Efficient egress by T. gondii critically relies on micronemal secretion of TgPLP1, a member of the membrane attack complex/perforin (MACPF) protein family. The domain arrangement for TgPLP1 includes a central MACPF domain that is flanked by an N-terminal domain (NTD) and a C-terminal domain (CTD). Both the NTD and CTD have membrane-binding activity, but only CTD is crucial for proper TgPLP1 function. The CTD includes the apicomplexan specific APCβ domain, which consists of 3 direct repeats with 4 highly conserved cysteines in each repeat and a C-terminal tail (CTT) that includes a basic patch.

Despite using a construct that encompassed the entire CTD, the resulting crystals contained only the APCβ domain. The TgPLP1 APCβ domain crystallized in the C121 space group with two monomers in the asymmetric unit. The structure was solved using iodine soaks and single-wavelength anomalous dispersion and subsequently refined to 1.13 Å resolution. The TgPLP1 APCβ structure shows that the β-rich repeat region is comprised of a single globular domain with internal pseudo threefold symmetry wherein each β-rich repeat forms a subdomain. Each of the three subdomains contains an internal antiparallel β-sheet and an outer β-hairpin. The inner and outer layers of each subdomain are held together, in part, by two disulfide bonds between the highly conserved cysteines. Subdomain 3 (S2C Fig blue), however, aligns less well with subdomain 1 (RMSD 3.207 Å) and subdomain 2 (RMSD 3.175 Å), with the majority of the alignment differences attributed to two loops that protrude from the “bottom” of subdomain 3. The longer of the two loops has hydrophobic character, and thus is termed the hydrophobic loop (colored cyan), whereas the shorter of the two loops has basic character, termed the basic loop (colored orange). Given the hydrophobic character of the loop at the bottom of the APCβ structure we reasoned that this loop has the potential to insert into the membrane upon binding. Thus, we conclude that the tryptophan located at the tip of the protruding hydrophobic loop is probably responsible for changes in the fluorescence spectra reported here.

>SNAVGLTPQDLSALTGVTRNLPKQLTQATQVAWSGPPPGFAKCPGGQVVILGFAMHLNFKEPGTDNFRIISCPPGREKCDGVGTASSETDEGRIYILCGEEPINEIQQVVAESPAHAGASVLEASCPDETVVVGGFGISVRGGSDGLDSFSIESCTTGQTICTKAPTRGSEKNFLWMMCVDKQYPGLRELVNVAELGSHGNANKRAVNSDGNVDVKCPANSSIVLGYVMEAHTNMQFVRDKFLQCPENASECKMTGKGVDHGMLWLFDRHALFGWIICKTVNEPAMHVATDVGKAKGNGKKKKGRKGKNKTNAPNEVEEGQQLGADSPSQVSVPADADSGPTSKTMSSLKLAPVKLLDL[2x]> MAHHHHHHMESLTLQPIARVEGTVN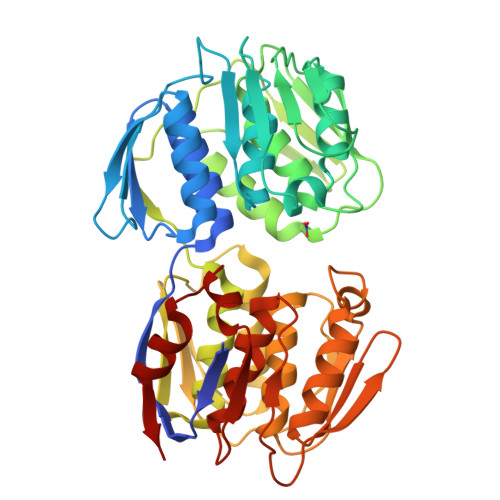LPGSKSVSNRALLLAALARGTTVLTNLLDSDDVRHMLNALSALGVQYTLSADRTRCEVTGNGGPLRSAAALELFLGNAGTAMRPLAAALCLGSNDIVLTGEPRMKERPIGHLVDALRQGGAQIDCLEQENYPPLRLRGGFQGGNVEVDGSVSSQFLTALLMTAPLAPQDTVIVIKGDLVSKPYIDITLHLMKTFGVEVDNQSYQRFVVRGKQQYQSPGDYLVEGDASSASYFLAAGAIKGGTVKVTGIGRNSVQGDIRFADVLEKMGATVTWGDDFIACTHGELKAVDMDMNHIPDAAMTIATAALFAQGTTTLRNIYNWRVKETDRLFAMATELRKVGAEVEEGEDYIRITPPAKLKYAEIGTYNDHRMAMCFSLVALSDTPVTILDPKCTAKTFPDYFEQLARISTLA4-(2-cyclopropylethylidene)-9-(1H-pyrazol-4-yl)-6-{[(1R)-1,2,2-trimethylpropyl]amino}benzo[c][1,6]naphthyridin-1(4H)-one 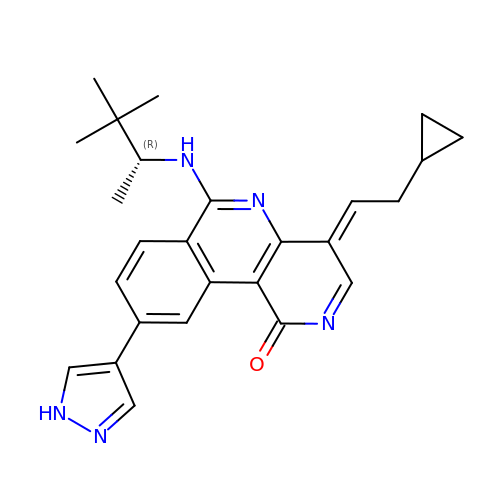| C26 H29 N5 O | LURVNNDHOKNBEC-RIEVCORGSA-N> RNLLELCQIDTIMEVNNLTTNEATPMERLRIPVQVQTQSGELCAAFKADPGLDGPW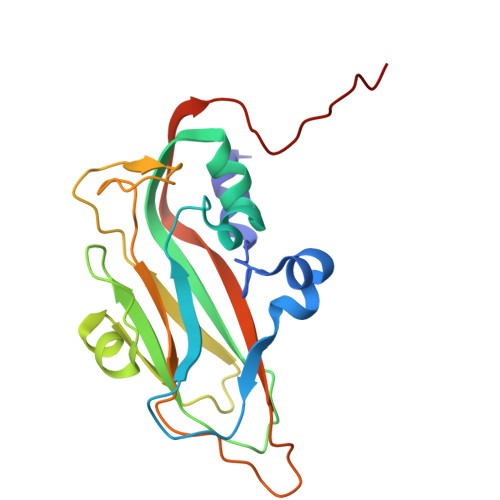QSTMVGQLCRYYTQWSGSLKITFMFTGSFMATGKMLIAYTPPGGSLPANRMQAMLGTHVIWDFGLQSSVTLVVPWISNTHYRSQATGSFFDYYATGIVSLWYQTNFVVPIGAPTTAYIVVLGSAQKNFTMRLCRDTSELTQAAEYQ>[3x]QIAALE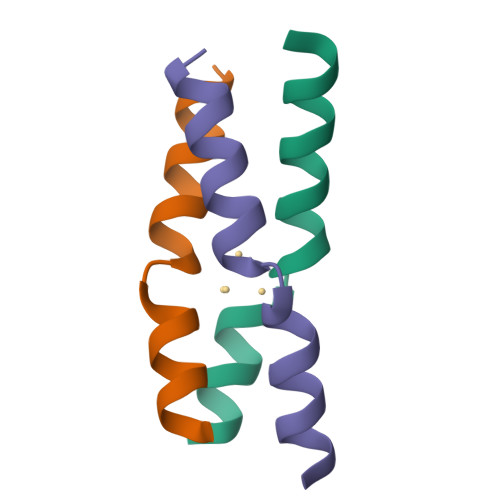QKIAALEQKCAACEQKIAALEQKGGY> LPRETDEEPEEPGKKGSFVEMVDNLRGKSGQGYYVEMTVGSPPQTLNILVDTGSSNFAVGAAPHPFLHRYYQRQLSSTYRDLRKGVYVPYTQGKWEGELGTDLVSIPHGPNVTVRANIAAITESDKFFINGSNWEGILGLAYAEIARPDDSLEPFFDSLVKQTHVPNLFSLQLCGAGFPLNQSEVLASVGGSMIIGGIDHSLYTGSLWYTPIRREWYYEVIIVRVEINGQDLKMDCKEYNYDKSIVDSGTTNLRLPKKVFEAAVKSIKAASSTEKFPDGFWL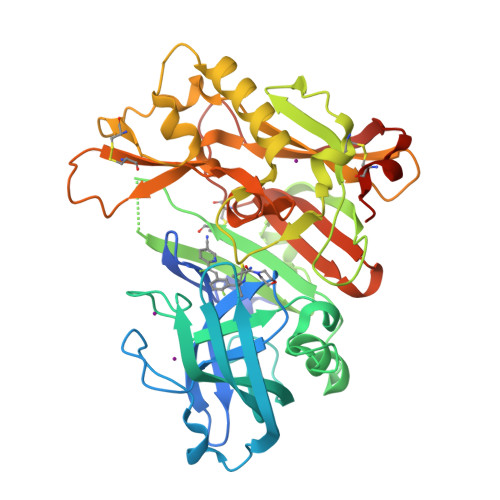GEQLVCWQAGTTPWNIFPVISLYLMGEVTNQSFRITILPQQYLRPVEDVATSQDDCYKFAISQSSTGTVMGAVIMEGFYVVFDRARKRIGFAVSACHVHDEFRTAAVEGPFVTLDMEDCGYNIPQTDES>[2x]SSIFLLSNVSEDAAQLAEELVREISKKEGTEVRFEKDDGFLTIEVKNLSEERLREIAKALQLIVDVANAERVVRERPGSNLAKK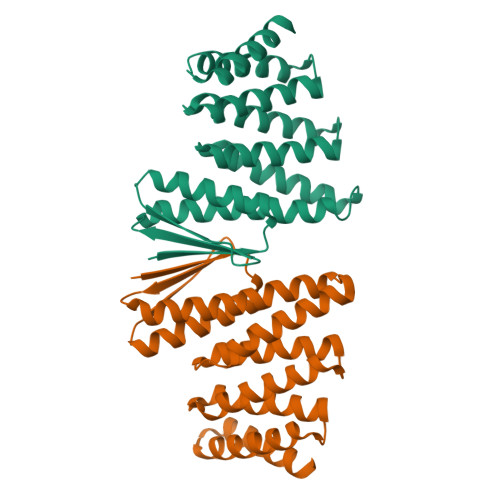ALEIILRAAEELAKLDLKASLKAAVRAAEKVVREQPGSNLAKKALEIILRAAEELAKLPDPEALKEAVKAAEKVVREQPGSELAKKALEIIERAAEELKKSPDPEAQKEAKKAEQKVREERPGS;>[2x]TWQWVLINISEEARQLIEKAVRAISKKEGTEVHFEKDDGVLHIRVKNLHEKRAREIHKVAKLILEVAAAERIVRERPGSNLAKKALEIILRAAEELAKADVDAALEAAVRAAEKVVREQPGSNLAKKALEIILRAAEELAKLPDPEALKEAVKAAEKVVREQPGSELAKKALEIIERAAEELKKSPDPEAQKEAKKAEQKVREERPGS> MPAPHGLSPLSKAFLMRRAFQRRILPHSLAMALSLPLAGYVQAQEVEFDIPPQALGSALQEFGRQADIQVLYRPEEVRNKRSSAIKGKLEPNQAITELLRGTGASVDFQGNAITISVAEAADSSVDLGATMITSNQLGTITEDSGSYTPGTIATATRLVLTPRETPQSITVVTRQNMDDFGLNNIDDVMRHTPGITVSAYDTDRNNYYARGFSINNFQYDGIPSTARNVGYSAGNTLSDMAIYDRVEVLKGATGLLTGAGSLGATINLIRKKPTHEFKGHVELGAGSW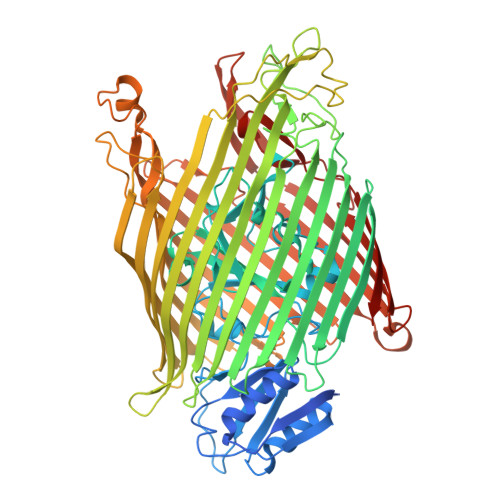DNYRSELDVSGPLTESGNVRGRAVAAYQDKHSFMDHYERKTSVYYGILEFDLNPDTMLTVGADYQDNDPKGSGWSGSFPLFDSQGNRNDVSRSFNNGAKWSSWEQYTRTVFANLEHNFANGWVGKVQLDHKINGYHAPLGAIMGDWPAPDNSAKIVAQKYTGETKSNSLDIYLTGPFQFLGREHELVVGTSASFSHWEGKSYWNLRNYDNTTDDFINWDGDIGKPDWGTPSQYIDDKTRQLGSYMTARFNVTDDLNLFLGGRVVDYRVTGLNPTIRESGRFIPYVGAVYDLNDTYSVYASYTDIFMPQDSWYRDSSNKLLEPDEGQNYEIGIKGEYLDGRLNTSLAYFEIHEENRAEEDALYNSKPTNPAITYAYKGIKAKTKGYEAEISGELAPGWQVQAGYTHKIIRDDSGKKVSTWEPQDQLSLYTSYKFKGALDKLTVGGGARWQGKSWQMVYNNPRSRWEKFSQEDYWLVDLMARYQITDKLSASVNVNNVFDKTYYTNIGFYTSASYGDPRNLMFSTRWDF>[2x]MTAQYQVQDGVAVITLDNPPVNGLGHSTRLGIVEGMTRALDDAAVKAIVITGAGKAFSGGADIREFNTPKAMQEPTLHSVIRVLEGSSKPVVAAVHSVAMGGGLELALGCNYRVASKGAQIALPEVKLGLLPGAGGTQRLPR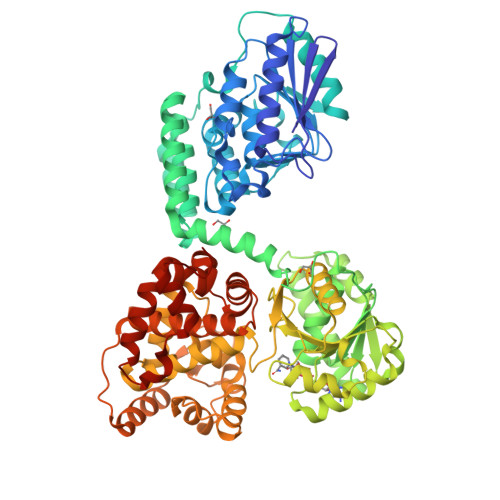VIGLEAAANMIVSGTPVLSEKFAGTKLFDEIVDGDVLPAAVKFAQNVGAATGPHPKVRDLKVRHENPEGYLGFARNTVAAMAKNFPAPLKCLEAVAGSLKPFEQGLKQEREGFLYLVTTPESRALRHAFFGERAASKIPDVPEGTPTRKIEKVAVIGAGTMGGGISMNFLNAGIPVTILETKQEALDRGVGIIRKNYENSAKKGKLTQEKVEQRMGLLSTTLSYDDLKDADLIIEAVFEEMGVKETVFKKLDEVAKQGAILASNTSTLDVNKIASFTKRPQDVVGMHFFSPANVMKLLEVVRGEKTGKDVLATVMQVGKKIKKTAVVSGVCDGFIGNRMIEQYSRQAGYLLDEGALPEQVDKAIEKFGFAMGPFRMGDLAGNDIGWAIRKRRAVDKPEIQYSKTADLLCEMGRFGQKTGAGWYDYKAGDRKPYPNQQVNDMIVQHSKDLGITRRKISDEEIVERLVFALVNEGARILEEGIASKASDIDMVYLTGYGFPLFRGGPMLYADQVGLYNVALSMKRYAKGYHGEAWQVAPLLQKLADEGKGFNGLEHHHHHH>MVDLPVIQPRLCTHARWPAPVYGLLVDPSLPSNPQWQNGRVHVDGTLLGTTPISGSWVSCFAAEAAYKFQSGTGEVATFTLIEQDGSAYVPGDRAAPLGYPDFSGQLEIEVQTETTKTGDKLKVTTFEMILGPTTNADQAPYQGRVFASVTAAASLDLVDGRVRAVPRSIYGFQDTIPEYNDGLLVPLAPPIGPFLPGEVLLRFRTYMRQIDTADAAAEAIDCALPQEFVSWFASNAFTVQSEALLLRYRNTLTGQLLFECKLYNEGYIALSYSGSGPLTFPTDGIFEVVSWVPRLYQLASVG[2x];>MEDPVTGPEEVSGQEQGSLTVQCRYTSGWKDYKKYWCQGVPQRSCKTLVETDASEQLVKKNRVSIRDNQRDFIFTVTM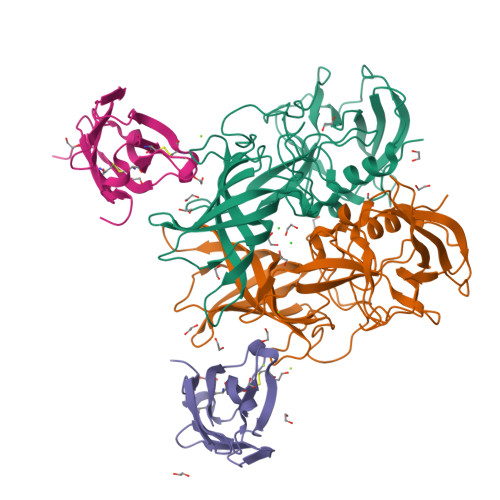EDLRMSDAGIYWCGITKGGLDPMFKVTVNIGPVPT[2x]> QIIGTVPGVEVGDEFQYRMELNLLGIHRPSQSGIDYMKDDGGELVATSIV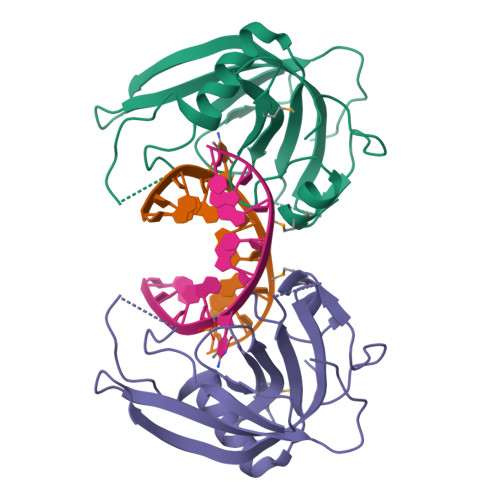SSGGYNDVLDNSDVLIYTGQGGNVGKKKNNEPPKDQQLVTGNLALKNSINKKNPVRVIRGIKNTTLQSSVVAKNYVYDGLYLVEEYWEETGSHGKLVFKFKLRRIPGQPELPWKEVA>SFKDLNLTDAQKQQIREIMKGQRDQMKRPPLEERRAMHDIIASDTFDKVKAEAQIAKMEEQRKANMLAHMETQNKI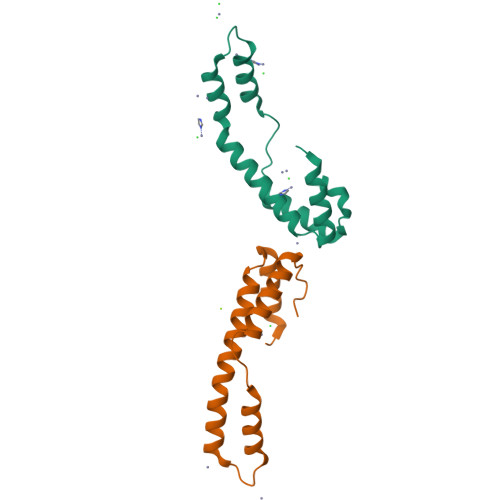YNILTPEQKKQFNANFEKRLT[2x]>SMDRIIEKLDHGWWVVSHEQKLWLPKGELPYGEAANFDLVGQRALQIGEWQGEPVWLVQQQRRHDMGSVRQVIDLDVGLFQLAGRGVQLAEFYRSHKYCGYCGHEMYPSKTEWAMLCSHCRERYYPQIAPCIIVAIRRDDSILLAQHTRHRNGVHTVLAGFVEVGET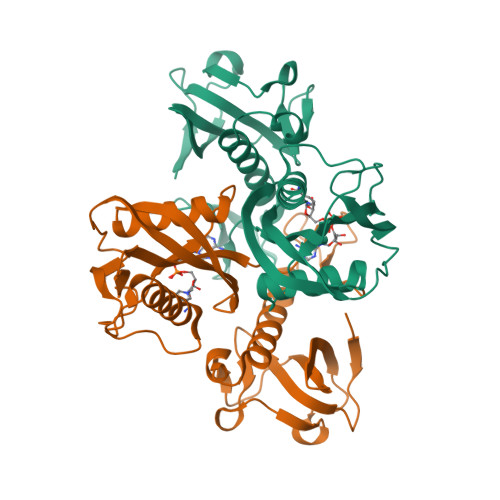LEQAVAREVMEESGIKVKNLRYVTSQPWPFPQSLMTAFMAEYDSGDIVIDPKELLEANWYRYDDLPLLPPPGTVARRLIEDTVAMCRAEYE[2x]>[2x]MISNDIAIDLGTANTLIYQKGKGIVLNEPSVVALRNVGGRKVVHAVGIEAKQMLGRTPGHMEAIRPMRDGVIADFEVAEEMIKYFIRKVHNRKGSGNPKVIVCVPSGATAVERRAINDSCLNAGARRVGLIDEPMAAAIGAGLPIHEPTGSMVVDIGGGTTEVAVLSLSGIVYSRSVRVGGDKMDEAIISYMRRHHNLLIGETTAERIKKEIGTARAPADGEGLSIDVKGRDLMQGVPREVRISEKQAADALAEPVGQIVEAVKVALEATPPELADDIADKGIMLTGGGALLRGLDAEIRDHTGLPVTVADDPLSCVALGCGKVLEHPKWMKGVLESTLAGSHHHHHH

In non-spherical bacteria, the actin homologue MreB is essential for shape maintenance as depletion of MreB through genetic knockouts or MreB-targeted drug treatment results in misshapen cells that eventually lyse. The MreB fibres are attached to the cell membrane via a hydrophobic loop in Thermotoga maritima as well as Gram+ bacteria and via an additional N-terminal amphipathic helix in Gram− bacteria. Here, we demonstrate that MreB from Caulobacter crescentus forms pairs of antiparallel protofilaments as revealed by crystal structures, an architecture unprecedented among actin-like proteins. The crystal structure of Caulobacter MreB (ΔCcMreBdh) reveals the typical actin fold, containing two domains on either side of a nucleotide binding cleft (Kabsch and Holmes, 1995).

A single mutation in the intra-protofilament interface (S283D, ΔCcMreBdmh) renders the protein monomeric, as shown both by crystallography and by EM. An initial domain closure is observed upon binding of AMMPNP by the monomer. Monomeric CcMreB shows little structural movement between the ADP- and the ATP analogue AMPPNP-bound states with domains I and II overlapping with an RMSD of 1.58 and 0.57 Å, respectively. In the monomeric state, the active site residue E140 of MreB has moved away from the nucleotide by just 1 Å. But consequently, it can no longer coordinate the attacking water, which is absent in this structure, and thus renders the monomer inactive. In monomeric, AMPPNP-bound MreB, the catalytic E140 moves 1 Å away from the nucleotide and is no longer able to bind to the catalytic water (blue). (E) Superposition of AMPPNP-bound monomeric ΔCcMreBdmh (m_3, shown in blue) and AMPPNP-bound polymeric ΔCcMreBdh (d_3, shown in pink) reveals a propeller twist: closing of the nucleotide-binding cleft by the movement of subdomain IB towards subdomain IIB, accompanied by a twist of subdomain IA, resulting of flattening of the molecule. In the AMPPNP-bound monomer conformation, no catalytic water is present in CcMreB, whereas the catalytic water in monomeric AMPPNP-bound ParM has moved away from the ideal geometry, thus hampering hydrolysis.> MDVVSLDKPFMYFEEIDNELDYEPESANE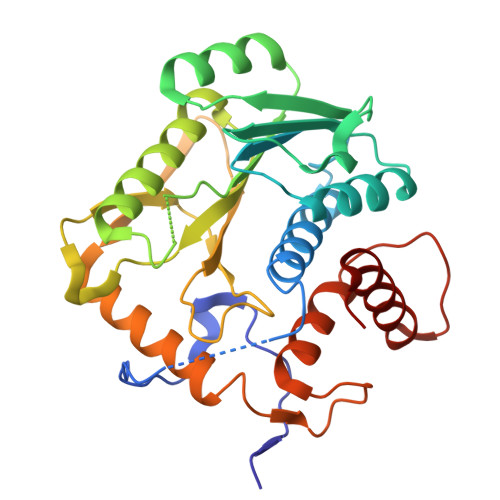VAKKLPYQGQLKLLLGELFFLSKLQRHGILDGATVVYIGSAPGTHIRYLRDHFYNLGVIIKWMLIDGRHHDPILNGLRDVTLVTRFVDEEYLRSIKKQLHPSKIILISDVASAAGGNEPSTADLLSNYALQNVMISILNPVASSLKWRCPFPDQWIKDFYIPHGNKMLQPFAPSYSAEMRLLSIYTGENMRLTRVTKSDAVNYEKKMYYLNKIVRNKVVVNFDYPNQEYDYFHMYFMLRTVYCNKTFPTTKAKVLFLQQSIFRFLNIP> IPCGESCVWLPCISSAIGCSCKSKVC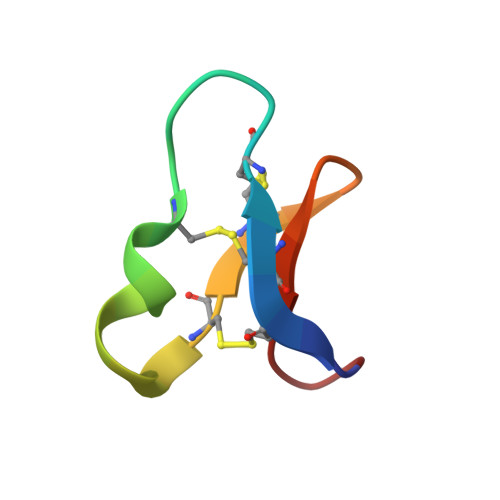YRNG> MHAVSVGKGSYATEFPEIDFGGINDPGFRDQQGEPPATIYRSDRVTGPMQTNSWWGSLAVDRFSMNQYPHPFSVRHRAEGLHVFYDAPHNMVVHENREAGTWHIHGAIGTDFTIKHSGTANFEQAVVDDYNDWYVRGLLENGAHQMAITYGVGSPYIFVEYEDGSAVLDFDIAPDVWEMNGHVIGFSTHDHKHYAAFAPPGQNWSGIGSKTLTNNADYIAIAKLPEKDGNMLAKFEQYAYSVVRDAVADWTYDEATGTVTTTFEVTTEAKVQGAPDGTIFALYPHQYRHLASSSENQLLQNYQYEIIRGTMIGLEGKRFTTELTYPGVLPSLPDLGDYDRERLIGYLHDATSDYPTGSDTYELGKYIGKLATLAPIADQMGEYELAEQFRGELKDILEDWLQATNASGQLKGKNLFYYNENWGTILGYHAAHSSATRINDHHFHYGYFVKAAAEIARADQEWAKSENWGGMIDLLIRDFMADRDDDLFPYLRMFDPYSGNSWADGLATFDAGNNQESSSEAMHAWTNVILWAEATGNKALRDRAIYLYTTEMSAINEYFFDVHQEIFPEEYGPEIVTINWGGKMDHATWWN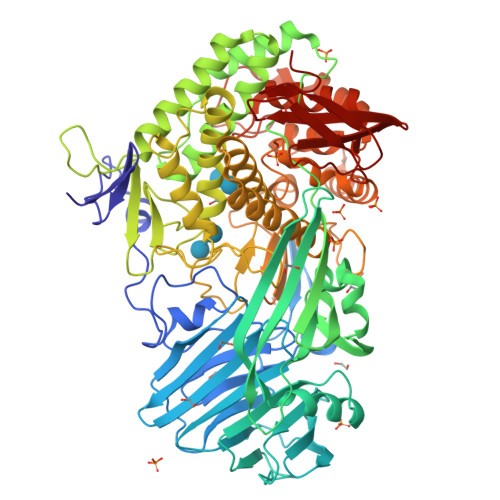SGKVEKYAINWLPFHGGSLYLGHHPDYVDRAYEELRRDIGSTDWNLWSNLVWMYRAFTNPDDALQQMEASIDDYGLFDPGNEKIIERGSTKAQTYHWIHNLAELGRVDPTVTANHPIYAVFNKNGNRTYIVYNFSDSPITVQFSDGHSIQVEPHSFNIGNG> MSTTTTEARSPLPLLLRRGRSSTALSASTAEARSPLSILQFRRRSSKDVRNITSVSSSLLPAFGTFIEDDNPSSKPFIVLHFDRRYRLWELFLVILVGYSAWASLFELAFEKAAEGALLTIDLVVDFFFAVDIILTFFVSYLDNTTYLNVTDHKLIAKRYLKSVAFVMDVASTLPIQFIYKTITGDVGRGQAFGFLNLLRLWRLRRVAELFKRLEKDAHFNYFVIRVIKLLCVTIFWIHLAGCILYWIAYHYPRPTDTWIGSQVEDFKERSVWLGYTYSMYWSIVTLTTVGYGDLHAVNSREKTFNMFYMLFNIGLTSY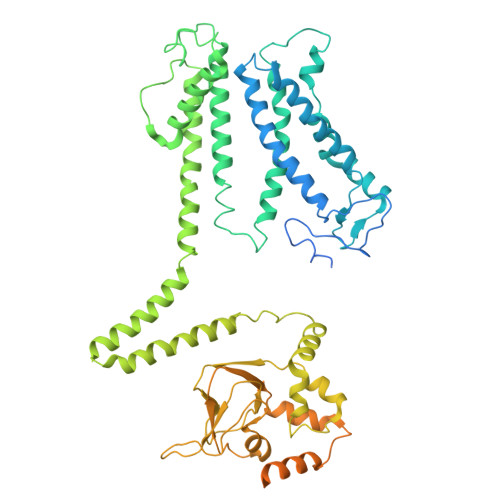IIGIMTNLVVHGALRTFAMRSAINDILRYTSKNRLPDTMREQMLAHMQLKFKTAELRQEEVLQDLPKAIRSSINQHLFRSIIEEAYLFKGFPEGLLVQLVSQIQAEYFPPKMEIILQNEIPTDFYVIVSGGVDIIASKGVSEQVLAKLGPGSMAGEIGVVFNIPQPFTVRTRRLSQVIRIGHHKFKEMVQSDNDVDAKMIIANFMTYLKGLNDELKKEIPFLRDLLDDADAQVQETVQSEETPQSNDEEIVTVSRHENGQIEERRREGVPKRVIIHGQAPPNQDNKNNGDSNGRLIILPDSIQLLFDLAEKKLGKRGSTIAMADGAHVEQIDALRENDHLYIF>[4x]MHTLYAPGGYDIMGYLIQIMNRPNPQVELGPVDTSCALILCDLKQKDTPIVYASEAFLYMTGYSNAEVLGRNC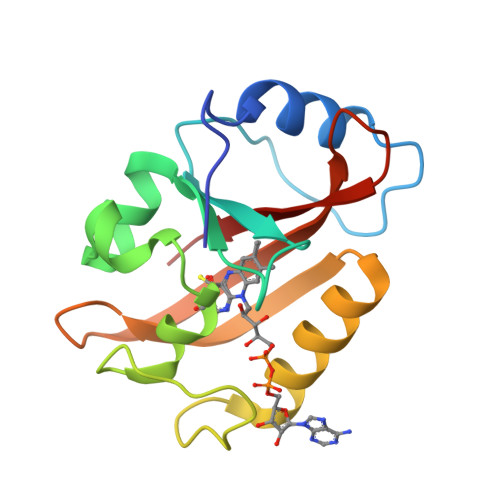RFLQSPDGMVKPKSTRKYVDSNTINTMRKAIDRNAEVQVEVVNFKKNGQRFVNFLTMIPVRDETGEYRYSMGFQCE> MGSDKIHHHHHHMKVKDVCKLISLKPTVVEEDTPIEEIVDRILEDPVTRTVY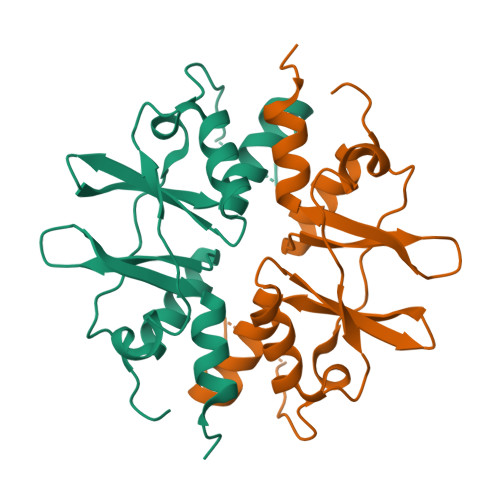VARDNKLVGMIPVMHLLKVSGFHFFGFIPKEELIRSSMKRLIAKNASEIMLDPVYVHMDTPLEEALKLMIDNNIQEMPVVDEKGEIVGDLNSLEILLALWKGREK>MVKLDTLDIFAVAPPPPGWGGRYWLLVRVTTDTGLTGLGEVYAAGVGPEAMTHVIHDVFTRHMRGEDPANIELMSRRAHSSGFTQRPDPTVFGAFSGLEMACWDILGKARDCPVWAMLGGKMNDRIRAYTYLYPEPHHDTNAFWTSPEMAAESAAARVAEGYTAVKFDPAGPYTMRGGHMPALSDIDLSARFCAAIRDAVGTQADLLFGTHGQFAPAGAIRLAKAIEPYDPLWYEEPIPPDNLPGLSEVAAHTSIPIATGERLTGVTEFTQALHHGARILQPALGRAGGIWEGKKIATLAAAFGAQLAPHLYAGPVEWAANVHLGVSCPNLLMVEAIETPFHEALVTGRPRVENGFVAAPDAPGLGITLNDAIANAHRYT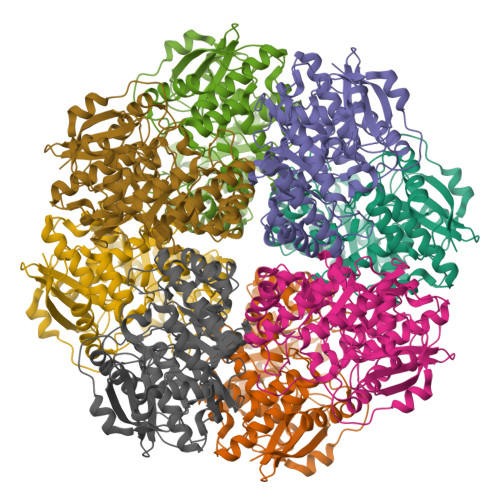GNRLHLEMQDAPCDWQNGNSFGGGAVDAENLYFQSHHHHHHWSHPQFEK[8x]>[2x]MHHHHHHSLLTEVETYVLSIVPSGPLKAEIAQRLEDVFAGKNTDLEVLMEWLKTRPILSPLTKGILGFVFTLTVPSERGLQRRRFVQNAL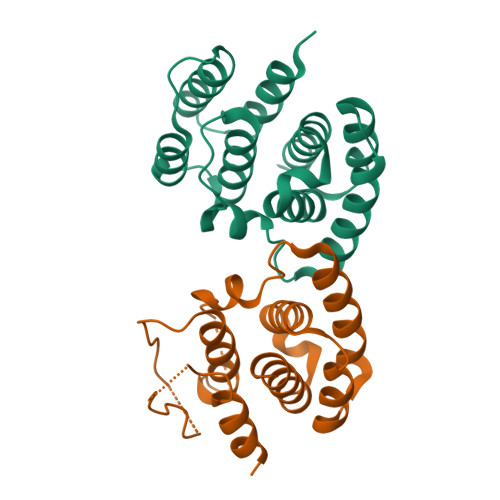NGNGDPNNMDKAVKLYRKLKREITFHGAKEIALSYSAGALASCMGLIYNRMGAVTTEVAFGLVCATCEQIADSQHRSHRQM>[2x]LKDLFRYIWPKGNNKVRIRVLIALGLLISAKILNVQVPFFFKQTIDSMNIAWDDPTVALPAAIGLTILCYGVARFGSVLFGELRNAVFAKVAQNAIRTVSLQTFQHLMKLDLGWHLSRQTGGLTRAMDRGTKGISQVLTAMVFHIIPISFEISVVCGILTYQFGASFAAITFSTMLLYSIFTIKTTAWRTHFRRDANKADNKAASVALDSLINFEAVKYFNNEKYLADKYNGSLMNYRDSQIKVSQSLAFLNSGQNLIFTTALTAMMYMGCTGVIGGNLTVGDLVLINQLVFQLSVPLNFLGSVYRDLKQSLIDMETLFKLRKNEVKIKNAERPLMLPENVPYDITFENVTFGYHPDRKILKNASFTIPAGWKTAIVGSSGSGKSTILKLVFRFYDPESGRILINGRDIKEYDIDALRKVIGVVPQDTPL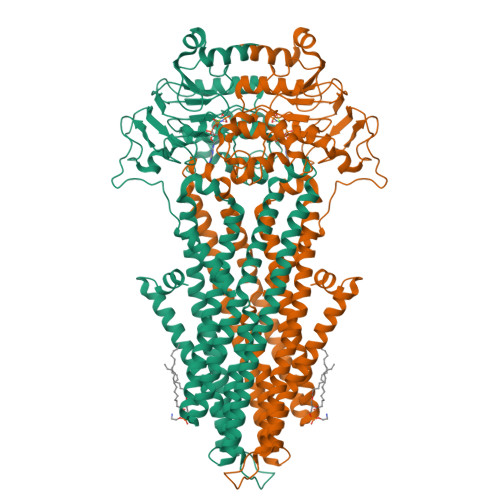FNDTIWENVKFGRIDATDEEVITVVEKAQLAPLIKKLPQGFDTIVGERGLMISGGEKQRLAIARVLLKNARIMFFDEATSALDTHTEQALLRTIRDNFTSGSRTSVYIAHRLRTIADADKIIVLDNGRVREEGKHLELLAMPGSLYRELWTIQEDLDHLENELKDQQELWSHPQFEK> MSVEVDKHRNTLQYHKKNPYSPLFSPISTYRCYPRVLNNPSESRRSASFSGIYKKRTNTSRFNYLNDRRVLSMEESMKDGSDRASKAGFIGGIRETLWNSGKYLWHTFVKNEPRNFDGSEVEA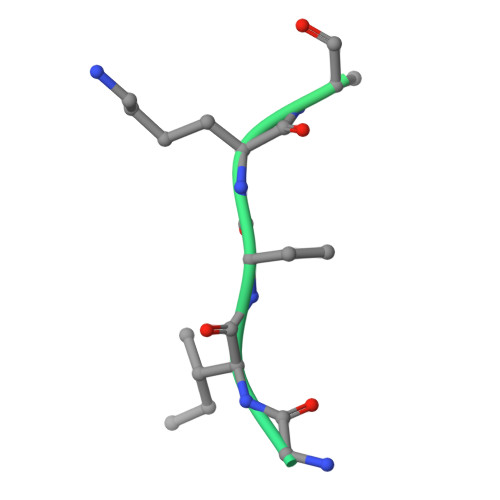SGNSDVESRSSGSRSSDVPYGLRENYS>GAMDPAVMKIEYYSQVLDMEWGVNVLYPDANRVEEPECEDIPVLYLLHGMSGNHNSWLKRTNVERLLRGTNLIVVMPNTSNGWYTDTQYGFDYYTALAEELPQVLKRFFPNMTSKREKTFI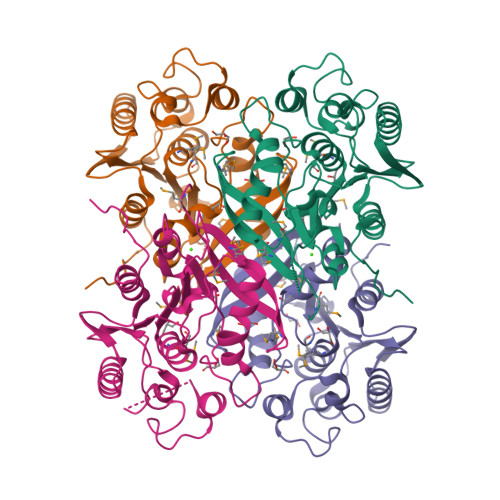AGLSMGGYGCFKLALTTNRFSHAASFSGALSFQNFSPESQNLGSPAYWRGVFGEIRDWTTSPYSLESLAKKSDKKTKLWAWCGEQDFLYEANNLAVKNLKKLGFDVTYSHSAGTHEWYYWEKQLEVFLTTLPIDFKLEERLT[4x]>MAHHHHHHVGTFENITAAPADPILGLADLFRADERPGKVDLGVGVYKDETGKTPVMTSVKKAEQYLLENETTKTYLGLDGLPEFGRCTQELLFGKGSALINDKRARTAQTPGGSGALRVAADFLAKNTSVKRVWVSNPTWPNHKAIFNSAGLEVREYAYYDAENHTLDFDALINSLNEAQAGDVVLFHGCCHNPTGADPTLEQWQTLAQLSVEKGWLPLIDIAYQGFGRGLEEDAEGLRAFAAMHKELIVASSCSKNFSLYNERVGACTLVAADSETVDRAFGQMKAAIRANYSNPPAHGASVVATILSNDALRAIWEQELTDMRQRIQRMRQLFVNTLQEKGANRDFSFIIKQNGMFSFSGLTKEQVLRLREEFGVYAVASGRINVAGMTPDNMAP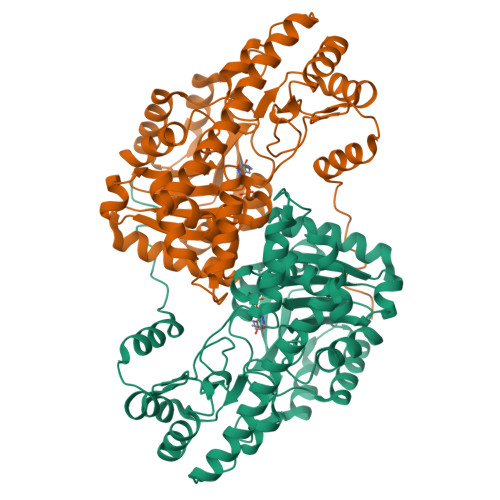LCEAIVAVL[2x]> SNYNQLKEDYNTLKRELSDRDDEVKRLRED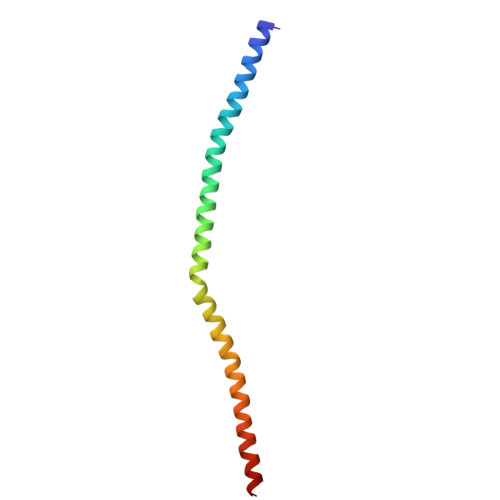IAKENELRTKAEEEADKLNKEVEDLTASLFDEANNMVADARKEKYAIEILNKRLTEQLREKDT> MK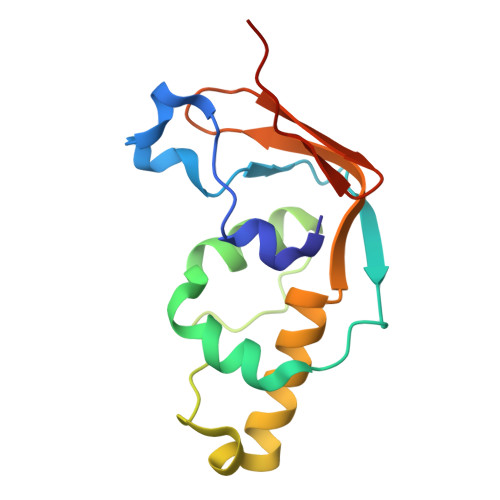FLTTNFLKCSVKACDTSNDNFPLQYDGSKCQLVQDESIEFNPEFLLNIVDRVDWPAVLTVAAELGNNALPPTKPSFPSSIQELTDDDMAILNDLHTLLLQTSIAEGEMKCRNCGHIYYIKNGIPNLLLPPHLV>MKLDIKKTFSNRSDRVKGIDFHPTEPWVLTTLYSGRVEIWNYETQVEVRSIQVTETPVRAGKFIARKNWIIVGSDDFRIRVFNYNTGEKVVDFEAHPDYIRSIAVHPTKPYVLSGSDDLTVKLWNWENNWALEQTFEGHEHFVMCVAFNPKDPSTFASGCLDRTVKVWSLGQSTPNFTLTTGQERGVNYVDYYPLPDKPYMITASDDLTIKIWDYQTKSCVATLEGHMSNVSFAVFHPTLPII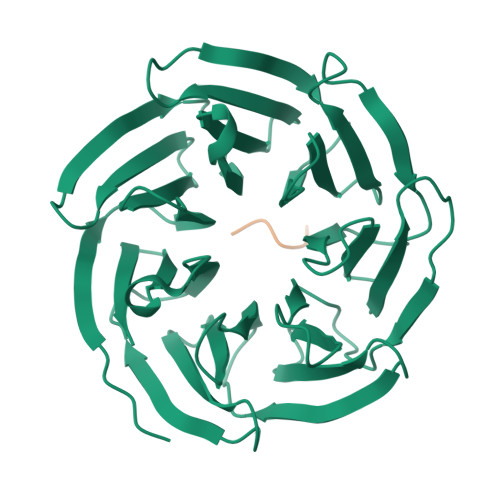ISGSEDGTLKIWNSSTYKVEKTLNVGLERSWCIATHPTGRKNYIASGFDNGFTVLSLG[2x];>[2x]ARKLD> SSSSESLSIIDVASDQNLFQTFIKEWRCKKRFSISLACEKIRGSGDDTLVVGLAVCWGGRDAYYFSLGGSGGLDPSLTLKDRMWYLQSCLRKESDKECSVVIYDFIQSYKILLLSCGISLEQSYEDPKVACWLLDPDSQEPTLHSIVTSFLPHELPLLEGMETSQGIQSLGLNAGSEHSGRYRASVESILIFNSMNQLNSLLQKENLQDVFRKVEMPSQYCLALLELNGIGFSTAECESQKHIMQAKLDAIETQAYQLAGHSFSFTSSDDIAEVLFLELKLPPGGSGGQFSTSKDVLNKLKALHPLPGLILEWRRITNAITKVVFPLQREKCLNPFLGMERIYPVSQSHTATGRITFTEPNIQNVPRDFEIKMGGSGGMPFSISMRHAFVPFPGGSILAADYSQLELRILAHLSHDRRLIQVLNTGADVFRSIAAEWKMIEPESVGDDLRQQAKQICYGIIYGMGAKSLGEQMGIKENDAACYIDSFKSRYTGINQFMTETVKNCKRDGFVQTILGRRRYLPGIKDNNPYRKAHAERQAINTIVQGSAADIVKIATVNIQKQLETFHSTFKSHGHREGMLQSDGGSGGCPIRGGFFILQLHDELLYEVAEEDVVQVAQIVKNEMESAVKLSVKLKVKVKIGASWGELKDFDV

The DNA damage response (DDR) protein DNA Polymerase θ (Polθ) is synthetic lethal with homologous recombination (HR) factors and is therefore a promising drug target in BRCA1/2 mutant cancers. Polθ is a unique DNA polymerase (Pol) and DNA helicase fusion protein that promotes multiple DNA repair mechanisms. The majority of Polθ’s DNA repair activities require it’s carboxy-terminal A-family DNA polymerase domain (Polθ-pol). For example, the DNA synthesis activity of Polθ is essential for its functions in MMEJ (TMEJ, Alt-EJ), translesion synthesis, and ssDNA gap repair.

A previously optimized highly soluble Polθ-pol construct (PolθΔL) was used for X-ray crystallography in which five short disordered loops were replaced with serine-glycine linkers. We conducted co-crystallization experiments using PolθΔL, along with RTX-152, DNA/DNA primer-template with a 5’ 10 nt ssDNA overhang, and incoming 2’,3’-dideoxyguanosine triphosphate (ddGTP). The structure of the resulting complex was determined to a resolution of 3.24 Å. The co-crystal structure of PolθΔL complexed with DNA/DNA, ddGTP, and RTx-152 shows the enzyme in the closed conformation with the inhibitor residing in an allosteric binding pocket located in the fingers domain of the polymerase. Within the binding pocket, RTx-152 forms hydrophobic contacts with many of the surrounding residues and a hydrogen bond with Y2420. Upon RTx-152 binding, Y2412 shifts its position to form pi stacking with the inhibitor, which in turn engages residues W2366 and M2402 to facilitate hydrophobic packing within the binding site. The pull of the N alpha helix towards the inhibitor brings E2365 closer to R2419, allowing for the formation of a salt bridge with a distance of 3.6 Å between the two residues. The salt bridge forms over the inhibitor and blocks its exit from the binding pocket. Intriguingly, the binding of RTx-152 to the closed conformation of PolθΔL appears to lock the enzyme into this state on the DNA/DNA, which likely prevents or slows the transition back to the open conformation which is required for subsequent nucleotide binding and addition cycles. This is due to the fact that the inhibitor occupies the same space as the N and O alpha helices during the open to closed conformation shift.>[4x]SNAEKSRSSWIKQLNASLDEIDPEVADIIELEKARQWKGFELIPSENFTSLSVMQAVGSVMTNKYSEGYPGARYYGGNEYIDMAETLCQKRALEAFQLDPSKWGVNVQSLSGSPANFQVYTALLKPHERIMALDLPHGGHLSHGYQTDTKKISAVSIFFETMPYRLD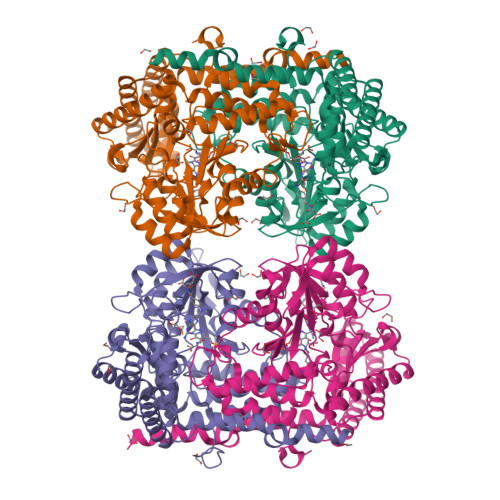ENTGYIDYDQLEKSAVLFRPKLIVAGASAYARLYDYARIRKVCNKQKAVMLADMAHISGLVAAGVIPSPFEYADVVTTTTHKSLRGPRGAMIFFRKGLKEINKQGKEVMYDYEDRINQAVFPGLQGGPHNHTITGLAVALKQARTPEYKAYQDQVLRNCSKFAETLLAKGYDLVSGGTDNHLVLVNLKNKGIDGSRVEKVLELVHIAANKNTVPGDVSAMVPGGIRMGTPALTSRGFIEEDFAKVAEYFDLAVKIALKIKAESQGTKLKDFVATMQSNEKLQSEMSKLREMVEEYAKQFPTIGFEKETMRYKE> SANNPWTGFQIFLSPYYANEVAAAAKQITDPTLSSKAASVANIPTFTWLDSVAKIPDLGTYLASASALGKSTGTKQLVQIVIYDLPDRDCAAKASNGEFSIANNGQANYENYIDQIVAQIQQFPDVRVVAVIEPDSLANLVTNLNVQKCANAKTTYLASVNYALTNLAKVGVYMYMDAGHAGWLGWPANLSPAAQLFTQVWQNAGKSPFIKGLATNVANYNALQAASPDPITQGNPNYDEIHYINALAPLLQQAGWDATFIVDQGKSGVQNIRQQWGDWCNIKGAGFGTRPTTNTGSQFIDSIVWVKPGGESDGTSNSSSPRYDSTCSLPDAA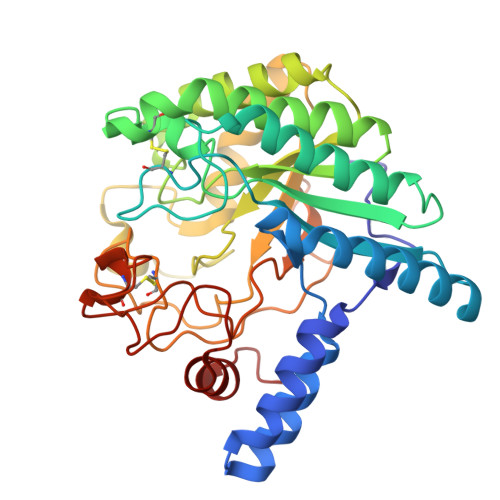QPAPEAGTWFQAYFQTLVSAANPPL>MNPFHELEPGPEVPEVVYALIEIPKGSRNKYEL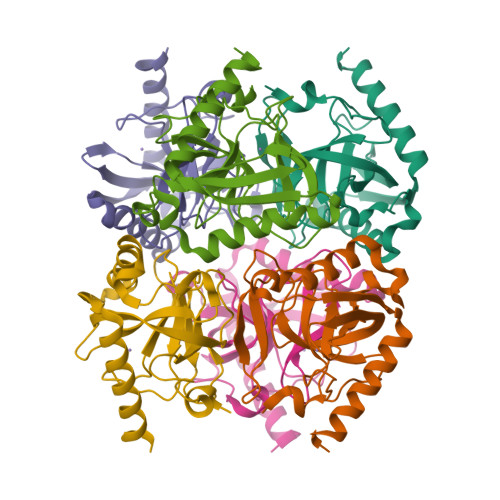DKKTGLLKLDRVLYSPFFYPVDYGIIPQTWYDDGDPFDIMVIMREPVYPLTIIEARPIGIMKMEDSGDKDWKVLAVPVEDPYFNDWKDISDVPKAFLDEIAHFFQRYKELQGKTTKIEGWGNAEEAKREILRAIEMYKEKFGKEE[2x]>GAPAAVDWRARGAVTAVKDQGQCGSCWAFSAIGNVECQWFLAGHPLTNLSEQMLVSCDKTDSGCSGGLMNNAFEWIVQENNGAVYTEDSYPYASGEGISPPCTTSGHTVGATITGHVELPQDEAQIAAWLAVNGPVAVAVDASSWMTYTGGVMTSC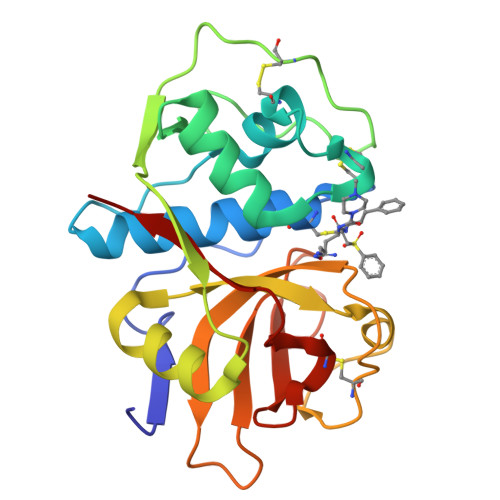VSEQLDHGVLLVGYNDSAAVPYWIIKNSWTTQWGEEGYIRIAKGSNQCLVKEEASSAVVG[2x]4-[(2,5-dioxo-2,5-dihydro-1H-imidazol-1-yl)methyl]-N-[2-(morpholin-4-yl)-1,3-benzothiazol-6-yl]benzamide 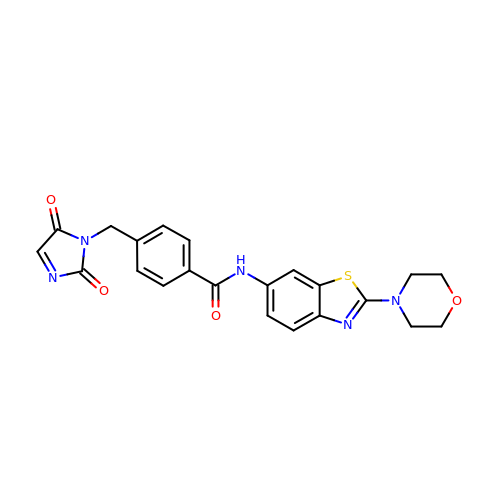| C22 H19 N5 O4 S | DIGDPYANABPQFC-UHFFFAOYSA-N>GMLEGLEAVRKRPGMYIGSTGERGLHHLIWEVVDNAVDEAMAGHATKVRVRLLADGGVEVSDDGRGIPVEMHESGVPTVDVVMTQVGVSVVNALSTRMEVEICRDGYQWFQTYDKSVPGTLKQGEKTRKTGTVVRF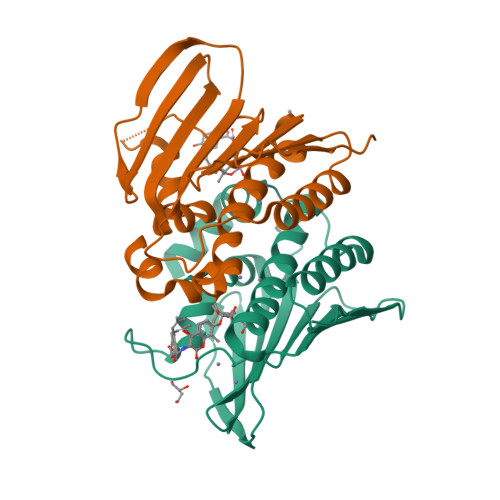WPDPDVFETTTFDFETVARRLQEQAFLNKGLTIELIDERDGKHRTFYYPG[2x]N-[3-(5-chloro-2-methoxyphenyl)-1-methyl-1H-pyrazol-4-yl]-2-methyl-2H-pyrazolo[4,3-c]pyridine-7-carboxamide | C19 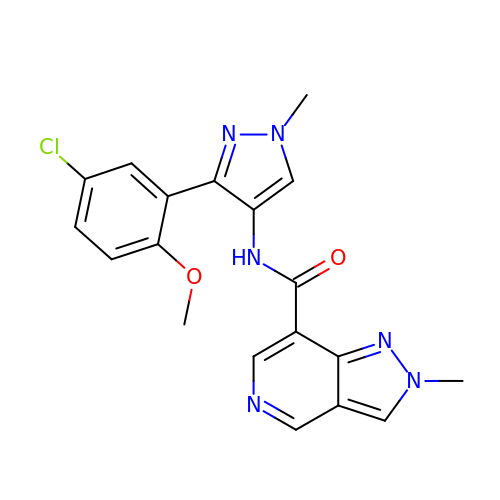H17 Cl N6 O2 | FCWWZBZYMGWKGY-UHFFFAOYSA-N>[2x]AHMNAGWVI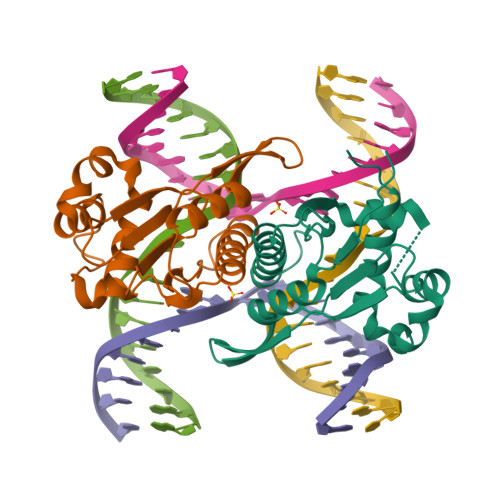GVAPDTSGALALLKPNQPPQVFDSPHLKVLVGKGVRKRLDAKAIVQLLKSFEAPIGTTVYVAQSTPYPQDGKQGWWSGGFGYGMWIGILVASGFSVIPVPSSAWKSEFQLTKERSNKDYSRQVASQLFPSLSSLLKRKKAHGRAAALLIAAYGKGIKINS2H-1,2,3-TRIAZOL-4-YLMETHANOL | C3 H5 N3 O | 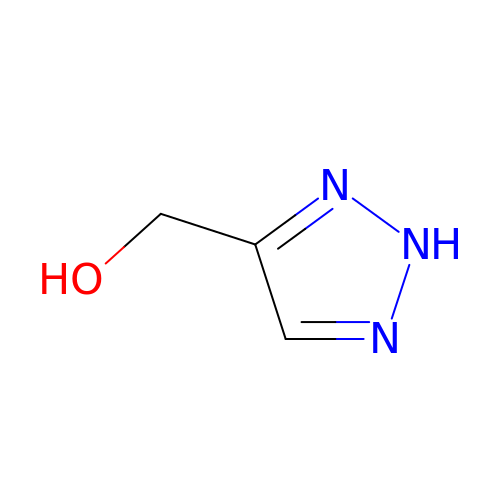OADYBXHYXPEGHX-UHFFFAOYSA-N>[2x]MNITPFPTLSPATIDAINVIGQWLAQDDFSGEVPYQADCVILAGNAVMPTIDAACKIARDQQIPLLISGGIGHSTTFLYSAIAQHPHYNTIRTTGRAEATILADIAHQFWHIPHEKIWIEDQSTNCGENARFSIALLNQAVERVHTAIVVQDPTMQRRTMATFRRMTGDNPDAPRWLSYPGFVPQLGNNADSVIFINQLQGLWPVERYL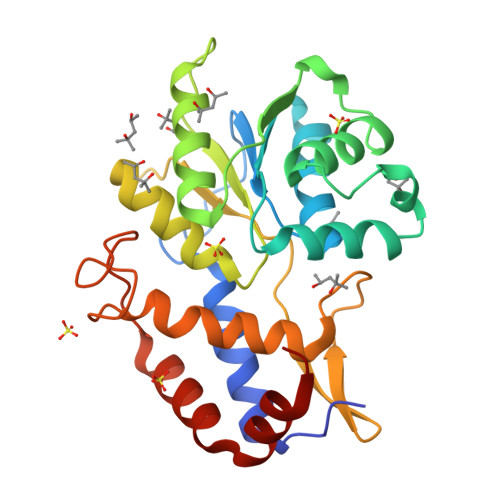SLLTGELPRLRDDSDGYGPRGRDFIVHVDFPAEVIHAWQTLKHDAVLIEAMESRSLR>[2x]MAEALFKEIDVNGDGAVSYEEVKAFVSKKRAIKNEQLLQLIFKSIDADGNGEIDQNEF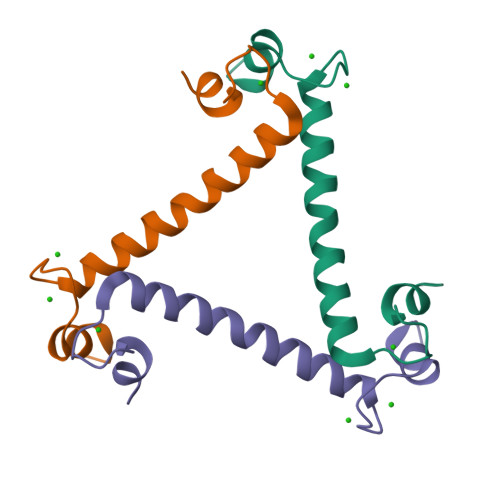AKFYGSIQGQDLSDDKIGLKVLYKLMDVDGDGKLTKEEVTSFFKKHGIEKVAEQVMKADANGDGYITLEEFLEFSL> HSNEKWFHGKLGAGRDGRHIAERLLTEYCIETGAPDGSFLVRESETFVGDYTLSFWRNGKVQHCRIHSRQDAGTPKFFLTDNLVFDSLYDLITHYQQVPLRCNEFEMRLSEPVPQTNAHESKEWYHASLTRAQAEHMLMRVPRDGAFLVRKRNEPNSYAISFRAEGKIKHCRVQQEGQTVMLGNSEFDSLVDLISYYEKHPLYRKMKLRYPINEEALEKIGTAEPDYG;>DDLYE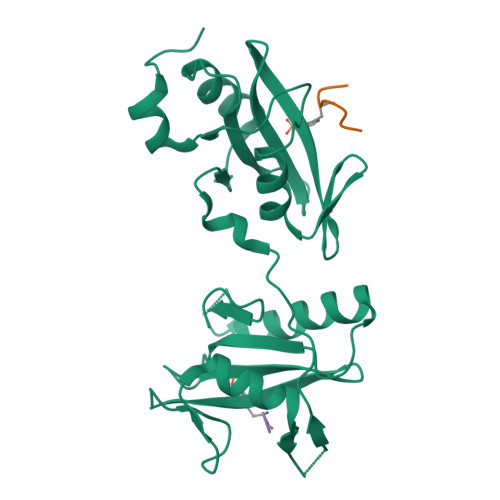EVLFPRN[2x]{2-[(2-chloro-6-fluorophenyl)amino]-5-methylphenyl}acetic 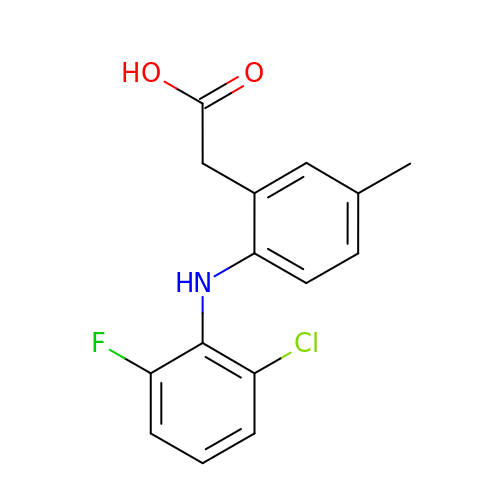acid | C15 H13 Cl F N O2 | KHPKQFYUPIUARC-UHFFFAOYSA-N>[6x]PPYTIVYFPVRGRCEAMRMLLADQGQSWKEEVVTIDTWMQGLLKPTCLYGQLPKFEDGDLTLYQSNAILRHLGRSLGLYGKNQREAAQMDMVNDGVEDLRGKY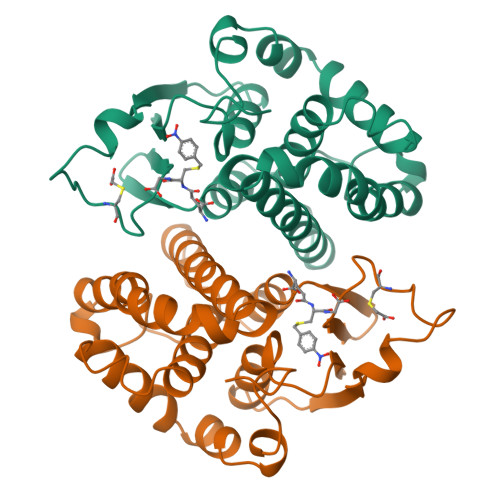VTLIYTNYENGKNDYVKALPGHLKPFETLLSQNQGGKAFIVGDQISFADYNLLDLLLIHQVLAPGCLDNFPLLSAYVARLSARPKIKAFLSSPEHVNRPINGNGKQ> GTNNGKQFIHNDTMEGGKLVCREIYAMNDAASGILNPVKMYKYSYDTDQQKTVKSTYAW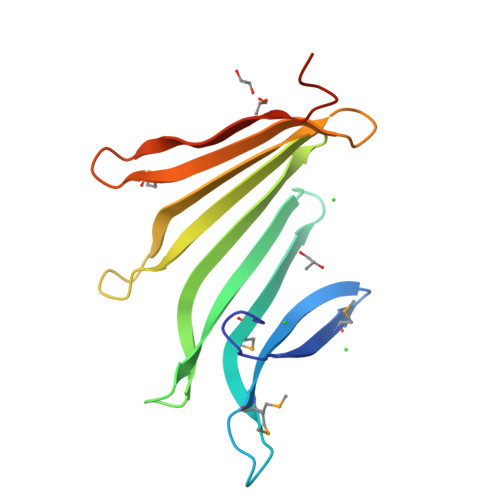NIFKNTWETESRTVISRYETETSVEYSVWNKEKGSFDLSKKYIYITDNNNQLIAQYAYKMNSRTNQWILEKDALTPIYENIYATTR Here, by solving the crystal structure, it is shown that MtGlu5 from Meiothermus taiwanensis WR-220, a GH5-family endo-β-1,4-glucanase (EC 3.2.1.4), has a bipartite architecture consisting of a Cel5A-like catalytic domain with a (β/α)8 TIM-barrel fold and an inserted CBM29-like noncatalytic domain with a β-jelly-roll fold. MtGlu5 contains a Cel5A-like CD similar to TmCel5A from Thermotoga maritima, but has an additional novel domain inserted into an internal site in the CD. Unlike other known cellulases with CBMs at the termini, this inserted CBM in the newly identified MtGlu5 acts in synergy with the CD, as demonstrated by ITC experiments.

Initial attempts to crystallize wild-type MtGlu5 failed. Instead, the inactive mutant E393Q (dubbed iMtGlu5) was first crystallized in a suitable form for structure determination. The CDs of two iMtGlu5 molecules were correctly located in the monoclinic P21 unit cell. The initial map showed some density outside the CD regions, and amino-acid residues corresponding to the CBM were manually placed, followed by computational refinement and new map calculations. Notably, the inserted CBM is not a fixed attachment, as its orientation varies with respect to the CD in the monoclinic and tetragonal crystals of iMtGlu5 and MtGlu5. The CBMs of the two iMtGlu5 molecules differ by a rigid-body rotation of 22.5°, and they differ from that of wild-type MtGlu5 by rotations of 25.3° and 10.8°. While large-scale conformational changes are often observed in enzymes upon substrate binding, the moderate flexibility of CBM in MtGlu5 probably allows switching between different orientations of polysaccharide chains. Because the CMC titrant and its molar concentration of binding sites are unknown, the n value was modified to 1 together with adjusting the concentration of the titrant. The data show that iMtGlu5 has a strong affinity for the recognition of long single polysaccharide chains with K d = 5.71 × 10−6.

>MGCQSTQLQTPAPDTGGIVELNRQLGRGVNLGNALEAPWEGAWGVRLEEGFFELIREAGFKTIRLPVSWTHHAGRAAPYTIDPAFFSRVDWAVTQATRRGLNIVVNVHHYDELNANPQAEEARYLSIWRQIAERYRNQPGSVYFELLNEPHGRFNDNPQLWNDLLAKALRVVRESNPSRAVIVGPVGWNSLWRLSELRLPDDPNLIVTFHYYDPLEFTHQGAEWLNPVPPTGVVWRENQGAFAAGWQNWSWGSRVGFVGEALEITYQEGWAGFYLHSDAGVEGYDRLAFRTSAPVSLQVSCRRDAPAKAVTTSGGVETVVNLSECGNPSRLTDLILQNNSPNARAAFRLERLELRGPGSPLALLTHQQNAIAQAMEFAQRWAEQNRRPIFVGQFGAYEKGDLDSRVRWTGAVRSELEKRNFSWAYWEFAAGFGIYDRTTRQWRTPLLKALVPEQPKLAAALEHHHHHH[2x]> SNA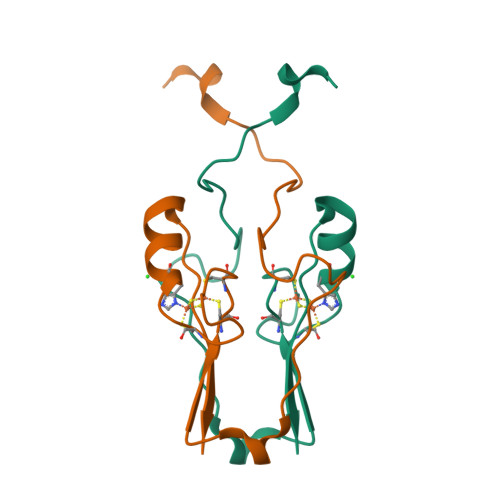RFYVKDHRNKAMINLHIQKDNPKIVHAFDMEDLGDKAVYCRCWRSKKFPFCDGAHTKHNEETGDNVGPLIIKKKET>[16x]XGEIAQALKEIAKALKEIAWAKKEIAQALKGX

αHBs are oligomers of 5 or more α-helical peptides that assemble into coiled-coil structures with central solvent-accessible channels. We targeted two properties of αHBs: oligomeric state, which directly affects the internal diameter of the channel; and the identities of channel-facing residues, which fine tune this dimension and introduce different chemistries. The αHBs are loaded with an environment sensitive dye (in this case, 1,6-diphenyl-1,3,5-hexatriene, DPH) that binds within the channels and fluoresces. Accordingly, challenging the array with analytes leads to differential displacement of the dye across the array to give a fluorescent fingerprint.

Despite the requirements for aliphatic residues at a and d, up to 40% of these can be changed to other side chains without compromising barrel integrity. We introduced mutations at one or two of these sites to generate four groups of αHB: Group I had entirely hydrophobic interiors, but with different sizes and shapes of channel; Groups II and III had polar uncharged or polar charged residues, respectively, at specific points along the channel; and Group IV had aromatic residues installed in their channels. The twelve Group III peptides had positively and negatively charged side chains, Lys and Glu, incorporated either singly or paired at a and d sites; and a single peptide with Asp at d. Finally, one third of the designs were crystallized and yielded 12 X-ray crystal structures, all of which were open αHBs with fully accessible channels. Focusing on the small molecules, the αSA signal from the more-polar AAs and CHOs is dominated by the polar and charged Group II and III αHBs.> GV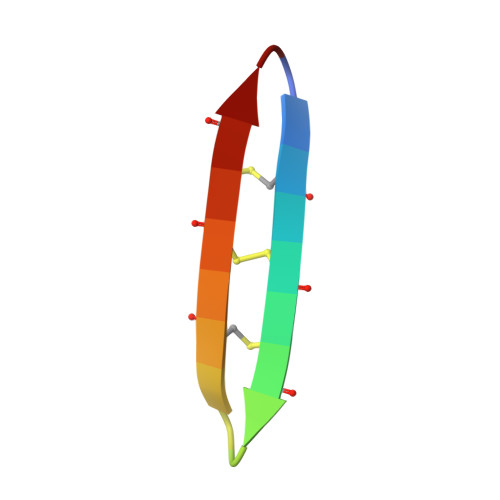CRCVCRRGVCRCVCRR Siroheme is the modified isobacteriochlorin tetrapyrrole used by siroheme-dependent sulfite and nitrite reductases (SiR/NiRs) in catalyzing the six-electron reduction of sulfite to sulfide or nitrite to ammonia. CysG is encoded by a gene fusion between a C-terminal SUMT (CysGA) and an N-terminal bifunctional dehydrogenase/ferrochelatase (CysGB). The N-terminal enzyme module, CysGB, is a three-domain bifunctional dehydrogenase/ATP-independent class III ferrochelatase12 that performs the final two steps of siroheme biosynthesis. The C-terminal enzyme module, CysGA, is homologous to a well-studied class of SAM-dependent uro’gen III methyltransferases (SUMTs) that catalyzes the methylations to generate precorrin-210,13.

D262 comes from the CysGA module, opposing D104 but adjacent to R260/R261 and sitting above the tetrapyrrole nitrogens. Therefore, we wanted to know if D262 from CysGA was important for catalysis, so we altered it to an alanine or an asparagine (D262A or D262N). No gross structural defects were apparent. Both complemented cysG deficiency, but the altered enzymes produced the fluorescent intermediate, with defects in the dehydrogenase and chelatase activities. D262N was more affected by increasing Co2+ than CysG. R261A, D262A, and D262N retain some activity for both chemistries. Given that both D262 variants retain activity, however, and its absence from Met8p, we conclude that in CysG, D262 is not strictly required. It does, however, interact with an arginine that directly binds the sirohydrochlorin, so helps form the active site to bind the tetrapyrrole in the correct orientation. P133G behaves similarly to D262N: strongly affected by increasing cobalt concentrations.

>[2x]MDHLPIFCQLRDRDCLIVGGGDVAERKARLLLEAGARLTVNALTFIPQFTVWANEGMLTLVEGPFDETLLDSCWLAIAATDDDTVNQRVSDAAESRRIFCNVVDAPKAASFIMPSIIDRSPLMVAVSAGGTSPVLARLLREKLESLLPQHLGQVARYAGQLRARVKKQFATMGERRRFWEKFFVNDRLAQSLANADEKAVNATTERLFSEPLDHRGEVVLVGAGPGDAGLLTLKGLQQIQQADIVVYDRLVSDDIMNLVRRNADRVFVGKRAGYHCVPQEEINQILLREAQKGKRVVRLKGGDPFIFGRGGEELETLCHAGIPFSVVPGITAASGCSAYSGIPLTHRDYAQSVRLVTGHLKTGGELDWENLAAEKQTLVFYMGLNQAATIQEKLIAFGMQADMPVALVENGTSVKQRVVHGVLTQLGELAQQVESPALIIVGRVVALRDKLNWFSNH>MGSSHHHHHHSSGLVPRGSVCMTEIATTSGARSVGLLSVGAYRPERVVTNDEICQHIDSSDEAIYTRTGIKTRRFAADDESAASMATEACRRALSNAGLSAADIDGVIVTTNTHFLQTPPAAPMVAASLGAKGILGFDLSAGCAGFGYALGAAADMIRGGGAATMLVVGTEKLSPTIDMYDAGNCFIFADGAAAVVVGETPFQGIGPTVAGSDGEQADAIRQDIDWITFAQNPSGPRPFVRLEGPAVFRWAAFKMGDVGRRAMDAAG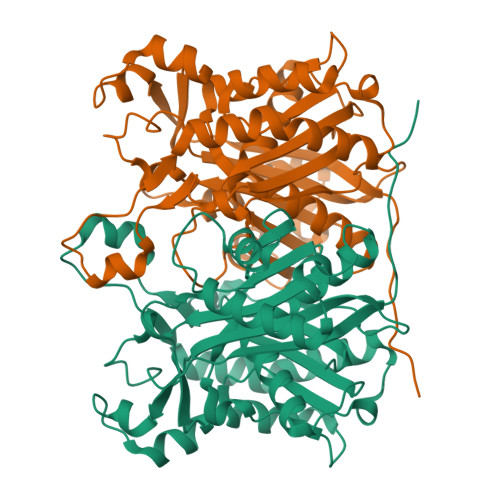VRPDQIDVFVPHQANSRINELLVKNLQLRPDAVVANDIEHTGNTSAASIPLAMAELLTTGAAKPGDLALLIGYGAGLSYAAQVVRMPKG[2x]>SAKGYVGDPSDEYYMVTFLSGIDYWKYCFEGFEDAAKAIGVTAKYTGQTDTDVSGQVAVLEQVIAQKPKGIAVTAVNSTALADTINSAIEQGISVVCFDSDSPTSNRSAYLGTGNYAAGQKAAEFLVPLVNYKGKIAVLYTVGAENSESRVQGFEDWCKQNAPEVSLVKVNDAGDTTVAADNLAA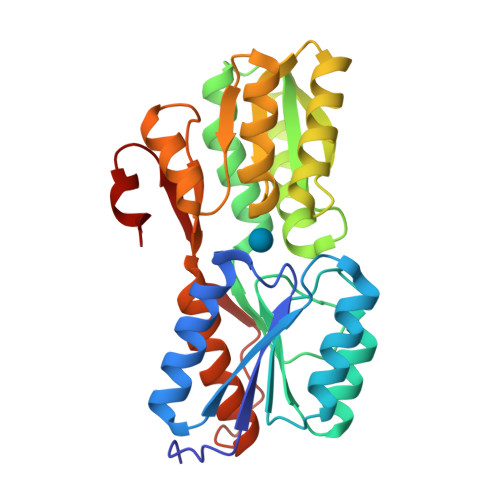ALQANDDIVGVFCVDGVAGTAGPTAVAESKKDLRVLAFDVDVTVLDKVKSGEIDGTVAQGMYNMGYWSLMMLYTEANGLSSKALPGNLDTGVVIVTKDNVDEYYPKK[4x]>EKDRKRILITGGAGFVGSHLTDKLMMDGHEVTVVDNFFTGRKRNVEHWIGHENFELINHDVVEPLYIEVDQIYHLASPASPPNYMYNPIKTLKTNTIGTLNMLGLAKRVGARLLLASTSEVYGDPEVHPQSEDYWGHVNPIGPRACYDEGKHVAETMCYAYMKQEGVEVRVARIFNTFGPRMHMNDGRVVSNFILQALQGEPLTVYGSGSQTRAFQYVSDLVNGLVALMNSNVSSPVNLGNPEEHTILEFAQLIKNLVGSGSEIQFLSEAQDDPQKRKPDIKKAKLMLGWEPVVPLEEGLNKAIHYFRKELEYQANNQYIPKPKPARI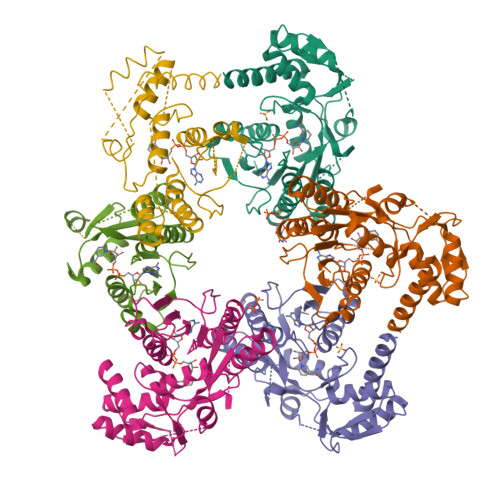KKGRTRHS[6x]>[4x]GPLGSNIEQYIHDLDSNSFELDLQFSEDEKRLLLEKQAGGNPWHQFVENNLILKMGPVDKRKGLFARRRQLLLTEGPHLYYVDPVNKVLKGEI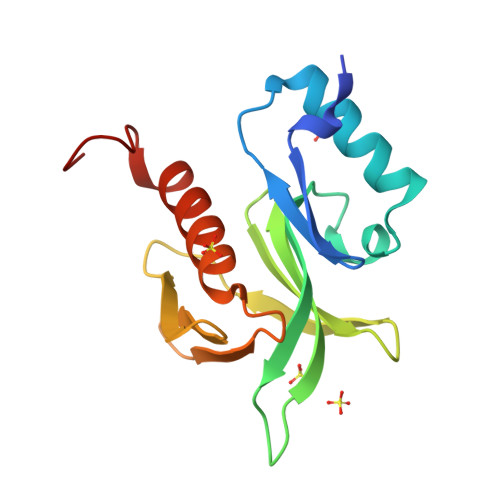PWSQELRPEAKNFKTFFVHTPNRTYYLMDPSGNAHKWCRKIQEVWRQRYQSHPDAAVQ>[2x]AMDPMKIADLMTLLDHHVPFSTAESWDNVGLLIGDEDVEVTGVLTALDCTLEVVNEAIEKGYNTIISHHPLIFKGVTSLKANGYGLIIRKLIQHDINLIAMHTNLDVNPHGVNMMLAKVMGLKNISIINNQQDVYYKVQTYIPKDNVGPFKDKLSENGLAQEGNYEYCFFESEGRGQFKPVGEANPTIGQIDKIEDVDEVKIEFMIDAYQKSRAEQLIKQYHPYETPVFDFIEIKQTSLYGLGVMAEVDNQMTLEDFAADIKSKLNIPSVRFVGESNQKIKRIAIIGGSGIGYEYQAVQQGADVFVTGDIKHHDALDAKIHGVNLIDINHYSEYVMKEGLKTLLMNWFNIEKINIDVEASTINTDPFQYI

SA1388 was predicted to contain a central PII-like domain and two flanking regions, which together belong to the NIF3-like protein family. Overall, the protein is organized into three distinct structural domains with interconnecting topological connectivities. The two NIF3 domains at the N- and C-terminus of the protein (henceforth denoted as NIF3-N and NIF3-C, respectively) have the same overall fold as canonical NIF3-like proteins, with a central 5 stranded mixed β-sheet and a pair of helices on either side. The middle region of the polypeptide (residues 126–236) bulges out between the two NIF3 domains and is structured as a classical PII-like fold with a (β/α/β)2 architecture, confirming our earlier prediction.

The final model of SA1388 (gi:54040095 Swissprot: P67273;) refined to 2.0Å resolution consists of two subunits in the asymmetric unit. The two SA1388 monomers in the asymmetric unit tightly associate to form a dimer along the sides of the two NIF3 domains opposite to where the PII-domain is located. The PII-like domain juts out of the dimer on the side opposite the dimer interface and forms homotrimers by interacting with the PII-like domains of symmetry related molecules along the three-fold axes. In SA1388, the two entries to the central hollow space are capped by the two PII domain trimers. We observe clear electron density for two tightly bound metal ions at the junction of the two NIF3 domains in each SA1388 monomer close to the protein surface that face inside the hexameric toroid. We have therefore modelled two zinc atoms at the putative active site. Both metal atoms are tethered to the protein through several histidine and aspartate residues. Residue Glu329 is coordinated to both metal ions, while a water molecule, or more likely a hydroxide ion, also bridges the two metal ions. Additionally, we observe a clear electron density for a ligand of unknown identity in close proximity to the two bound zinc atoms that would provide two additional metal ligands, one to each of the two metal ions to complete the octahedral metal center configuration. The contours of the difference electron density map after final refinement suggests the presence of a head group directly ligated to the metal ions and a mostly aliphatic tail that has few specific polar interactions with the surrounding protein residues.> PGVERTDITYNLTSDIDAAAYLEELKQNPIINNKIMNPVGQCESLMTPVSNFMNEKGFDNIRYRG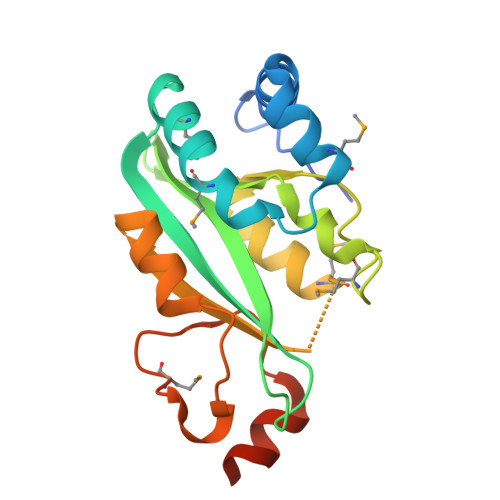IFIWDKPTEEIPTNHFAVVGNKEGKDYVFDVSAHQFENRGMSNLNGPLILSADEWVCKYRMATRRKLIYYTDFSNSSIAANAYDALPRELESESMAGKVFVTSPRWFNTFKKQKYSLIGKM> NPVERYVDEVLNEVLVVPNINQSHPTTSNAAPVLDAAETGHTNKIQPEDTIETRYVQSSQTLDEMSVESFLGRSGCIHESVLDIVDNYNDQSFTKWNINLQEMAQIRRKFEMFTYARFDSEITMVPSVAAKDGHIGHIVMQYMYVPPGAPIPTTRDDYAWQSGTNASVFWQHGQPFPRFSLPFLSIASAYY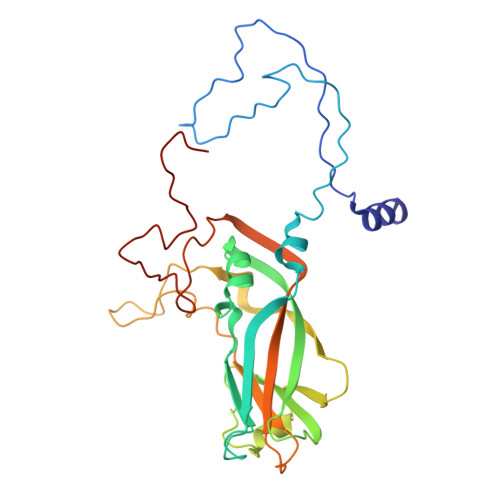MFYDGYDGDTYKSRYGTVVTNDMGTLCSRIVTSEQLHKVKVVTRIYHKAKHTKAWCPRPPRAVQYSHTHTTNYKLSSEVHNDVAIRPRTNLTTV>AADIFSKFKKDMEVKFAQEFGSNKQTGGDITDKTAKFLRLGPEQDPRKVEMIKAGKEIAEKRGIAFYNPMMHSGAPLGQRAITPYTISGTDIVCEPDDLHYVNNAAMQQMWDDIRRTCIVGLDMAHETLEKRLGKEVTPETINHYLEVLNHAMPGAAVVQEMMVETHPALVDDCYVKVFTGDDALADEIDKQFLIDINKEFSEEQAAQIKASIGKTSWQAIHIPTIVSRTTDGAQTSRWAAMQIGMSFISAYAMCAGEAAVADLSFAAKHAALVSMGEMLPARRARGPNEPGGLSFGHLSDIVQTSRVSEDPAKIALEVVGAGCMLYDQIWLGSYMSGGVGFTQYATAAYTDDILDNNTYYDVDYINDKYNGAATVGKDNKVKASLEVVKDIATESTLYGIETYEKFPTALEDHFGGSQRATVLAAAAGVACSLATGNANAGLSGWYLSMYLHKEAWGRLGFFGFDLQDQCGATNVLSYQGDEGLPDELRGPNYPNYAMNVGHQGGYAGIAQAAHSGRGDAFTVNPLLKVCFADDLLPFNFAEPRREFGRGAIREFVPAGERSLVIPAK[2x];>[2x]SDTVDIYDDRGKLLESNVDIMSLAPTRNAAIQSIIMDTKRSVAVNLAGIQGALASGKMGGKGRQILGRGLNYDIVGNADAIAENVKKLVQVDEGDDTNVIKVKGGKSLLIQSPKSRIIAGADFMSATTVGAAAVTQTIMDMFGTDPYDAPIVKSAVWGSYPQTMDLMGGQVQGILSIPQNNEGLGFSLRNIMANHVAAISNRNAMNASALSSIYEQSGIFEMGGAVGMFERHQLLGLAYQGLNANNLLYDIVKENGKDGTIGTVIESVVRRAIEAGIISVDKTAPSGYNFYKANDVPKWNACAAVGTLAATLVNCGAGRAAQNVSSTLLYFNDILEKETGLPGCDYGKVEGTAVGFSFFSHSIYGGGGPGVFNGNHVVTRHSRGFAIPCVCAAVALDAGTQMFSIESTSGLIGDVFGAIPEFREPIKAVAGVL;>[2x]AYERQYYPGATSVAANRRKHMSGKLEKLREISDEDLTAVLGHRAPGSDYPSTHPPLAEMGEPACSTRENVAATPGAAAGDRVRYIQFADSMYNAPATPYFRSYFAAINFRGVDPGTLSGRQ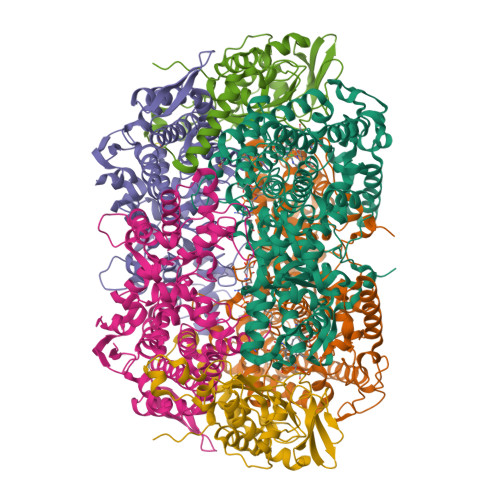IVEARERDMEQCAKVQMETEITDHALAGVRGATVHGHSVRLQEDGVMFDMLDRRRLENGTIIMDKDQVAIPLDRKVDLGKPMSSEEAAKRTTIYRVDNVAFRDDAEVVEWVHRIFDQRTKFGFQPK Two glycosyltransferases (GTases), SdgB and SdgA, are responsible for the glycosylation of S. aureus SDR proteins such as ClfA and ClfB. SdgB first appends N-acetyl­glucosamine (GlcNAc) moieties onto serine residues (O-glycosylation) within the SDR domain using uridine diphos­phate N-acetylglucosamine (UDP-GlcNAc) as a donor substrate. The subsequent addition of GlcNAc to the glycoproteins is catalyzed by the second enzyme, SdgA, yielding glycosylated SDR proteins in which each SD repeat is decorated with GlcNAc disaccharide moieties. The glycosylation of SDR proteins mediated by SdgA and SdgB protects SDR proteins from degradation by host proteases, thereby circumventing innate immune attack.

Despite the biological significance of these two glycosyltransferases involved in pathogenicity and avoidance of the host innate immune response, their structures and the molecular basis of their activity have not been investigated. This study reports the crystal structures of SdgB and SdgA from S. aureus as well as multiple structures of SdgB in complex with its substrates (for example UDP, N-acetylglucosamine or SDR peptides), products (glycosylated SDR peptides) or phosphate ions. In addition to the dimerization role, the inserted domain was found to serve as a binding platform for the SD repeats before and after glycosylation. Altogether, the extensive snapshots of SdgB complexes in multiple states provided a mechanistic insight into how SdgB recognizes and glycosylates the clustered serine residues in the SDR proteins.

>SMNYFVGNSLGVNLTGIEKAIINRLNLFKEMGRPAQCVFLSWNRYLYRNAQNYITSSDYINMYDFFQEATYLERNEPFDWLSYWTDECHYTLKHVENSHDFRIYDQERFLMYAHFQDPKYRILDYVNHFDSQRRKVKRDFYDVRGFLSCSRILVDKQQTLCEFFYNPEGDTKLEKYFSYKDGKPEVQKIIVYYANKQYFFNNETELGAFFIKQLYQHGDLFFSDRNVYTAPIFNLTPESIPVVAVLHSTHIKNIDALDSSPFKNVYKAMFENLSRYRAIIVSTEQQKLDVEKRINHTIPVVNIPVGYSETIDTPVQTLDQRSVKLISVARYSPEKQLHQQIELIKRLVSYVPKIELHMYGFGSESKKLNELIQKYGLENHVYLRGFLSNLDQEYSDAYLSLITSNMEGFSLALLESLAHGVPVISYDIKYGPNELITSDFNGYLITKNDEDALFDKVKYVIDHPEVQQRLSKGSLAKAQQYSKASLIKQWDQFVRLILEHHHHHH[2x];> DSD>[3x]GPGSMSEEMQPAVRVEKAGPVTTVILNRPHARNAVDGPTAAALLAAFTEFDADPEASVAVLWGDNGTFCAGADLKAMGTDRGNELHPHGPGPMGPSRLRLSKPVIAAISGHAVAGGIELALWCDLRVVEEDAVLGVFCRRWGVPLIDGGTIRLPRLIGHSRAMDLILTGRPVHANEALDIGLVNRVVARGQAREAAETLA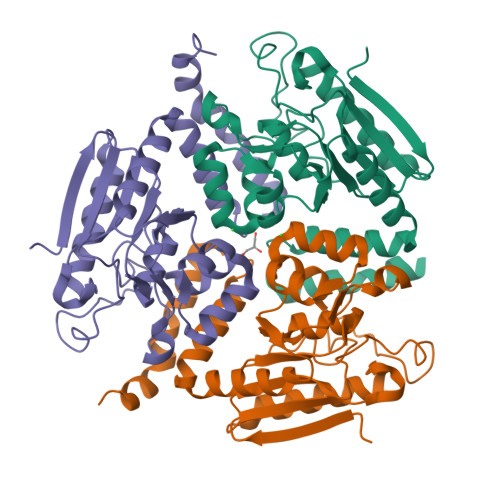AEIAAFPQQCVRADRDSAIAQWGMAEEAALDNEFGSIERVATEALEGAGRFAAGEGRHGAGV> GAMDGTAAEPRPGAGSLQHAQPPPQPRKKRPEDFKFGKILGEGSFSTVVLARELATSREYAIKILEKRHIIKENKVPYVTRERDVMSRLDHPFFVKLYFTFQDDEKLYFGLSYAKNGELLKYIRKIGSFDETCTRFYTAEIVSALEYLHGKGIIHRDLKPENILLNEDMHIQITDFGTAKVLSPESKQARANSFVGTAQYVSPELLTEKSACKSSDLWALGCIIYQLVAGLPPFRAGNEGLIFAKIIKLEYDFPEKFFPKARDLVEKLL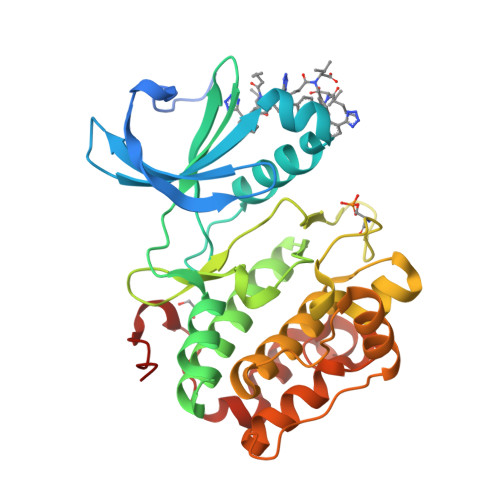VLDATKRLGCEEMEGYGPLKAHPFFESVTWENLHQQTPPKLT>SNAMVTTHDIKQWIETGLSESRVISAEGDGHHFEAVVLCPTFEGQTALTRH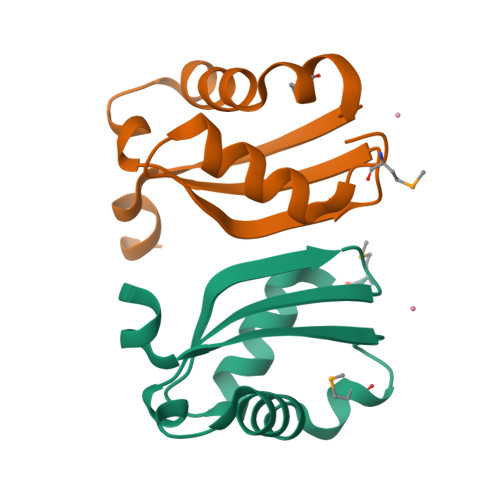RLVYNALGSHMQSDIHALSLKTYTPDEYERG[2x]ALLO-THREONINE | C4 H9 N O3 | 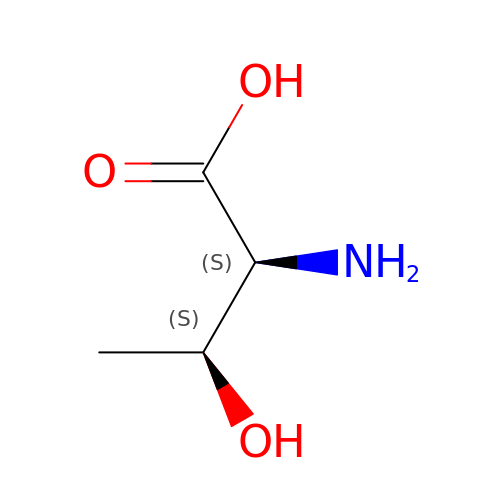AYFVYJQAPQTCCC-HRFVKAFMSA-N> MTVPSIVLNDGNSIPQLGYGVYKVPPADTQRAVEEALEVGYRHIDTAAIYGNEEGVGAAIAASGIARDDLFITTKLWNDRHDGDEPAAAIAESLAKLALDQVDLYLVHWPTPAADNYVHAWEKMIELRAAGLTRSIGVSNHLVPHLERIVAATGVVPAVNQIELHPAYQQREI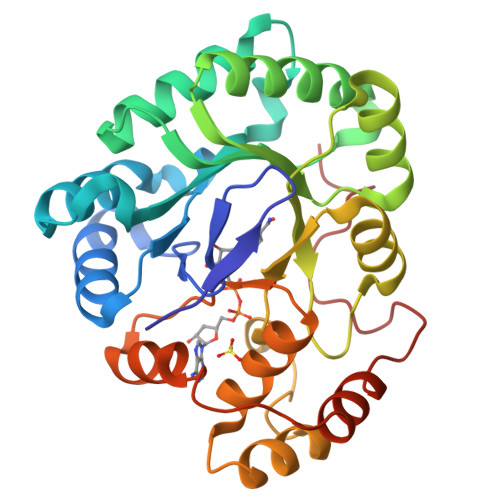TDWAAAHDVKIESWGPLGQGKYDLFGAEPVTAAAAAHGKTPAQAVLRWHLQKGFVVFPGSVRREHLEENLDVFDFDLTDTEIAAIDAMDPGDGSGRVSGHPDEVD> SDKIIHLTDDSFDTDVLKADGAILVDFWAEWCGRPCKMIAPILDEIADEYQGKLTVAKLNIDQNPGTAPKYGIRGI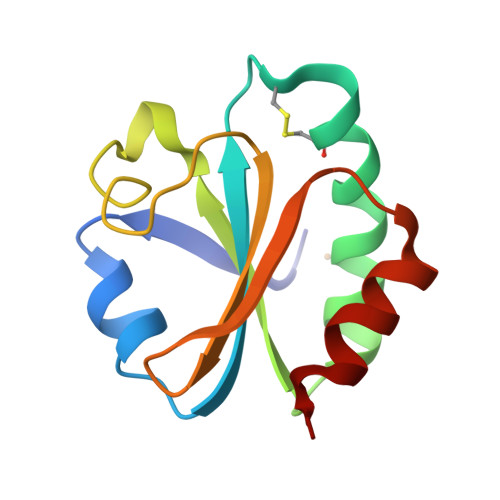PTLLLFKNGEVAATKVGALSKGQLKEFLDANLA>MKRNYILGLDIGITSVGYGIIDYETRDVIDAGVRLFKEANVENNEGRRSKRGARRLKRRRRHRIQRVKKLLFDYNLLTDHSELSGINPYEARVKGLSQKLSEEEFSAALLHLAKRRGVHNVNEVEEDTGNELSTKEQISRNSKALEEKYVAELQLERLKKDGEVRGSINRFKTSDYVKEAKQLLKVQKAYHQLDQSFIDTYIDLLETRRTYYEGPGEGSPFGWKDIKEWYEMLMGHCTYFPEELRSVKYAYNADLYNALNDLNNLVITRDENEKLEYYEKFQIIENVFKQKKKPTLKQIAKEILVNEEDIKGYRVTSTGKPEFTNLKVYHDIKDITARKEIIENAELLDQIAKILTIYQSSEDIQEELTNLNSELTQEEIEQISNLKGYTGTHNLSLKAINLILDELWHTNDNQIAIFNRLKLVPKKVDLSQQKEIPTTLVDDFILSPVVKRSFIQSIKVINAIIKKYGLPNDIIIELAREKNSKDAQKMINEMQKRNRQTNERIEEIIRTTGKENAKYLIEKIKLHDMQEGKCLYSLEAIPLEDLLNNPFNYEVDHIIPRSVSFDNSFNNKVLVKQEENSKKGNRTPFQYLSSSDSKISYETFKKHILNLAKGKGRISKTKKEYLLEERDINRFSVQKDFINRNLVDTRYATRGLMNLLRSYFRVNNLDVKVKSINGGFTSFLRRKWKFKKERNKGYKHHAEDALIIANADFIFKEWKKLDKAKKVMENQMFEEKQAESMPEIETEQEYKEIFITPHQIKHIKDFKDYKYSHRVDKKPNRELINDTLYSTRKDDKGNTLIVNNLNGLYDKDNDKLKKLINKSPEKLLMYHHDPQTYQKLKLIMEQYGDEKNPLYKYYEETGNYLTKYSKKDNGPVIKKIKYYGNKLNAHLDITDDYPNSRNKVVKLSLKPYRFDVYLDNGVYKFVTVKNLDVIKKENYYEVNSKCYEEAKKLKKISNQAEFIASFYNNDLIKINGELYRVIGVNNDLLNRIEVNMIDITYREYLENMNDKRPPRIIKTIASKTQSIKKYSTDILGNLYEVKSKKHPQIIKKG[2x];>SMRKTIERLLNSELSSNSIAVRTGV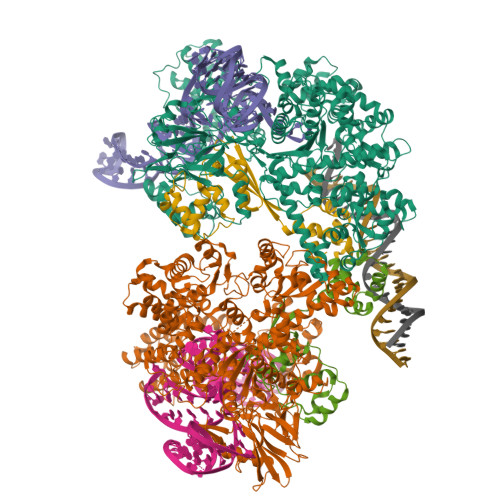SQAVISKLRNGKKELGNLTLNSAEKLFEYQKEMEKVDTWIVYRGRTADMNKSYIAEGSTYEEVYNNFVDKYGYDVLDEDIYEIQLLKKNGENLDDYDVDSDGINNYDKLDEFRESDYVDLEDYDYRELFENSSSQVYYHEFEITHE[2x]>MKYPPSLVSLIRELSRLPGIGPKSAQRLAFHLFEQPREDIERLASALLEAKRDLHVCPICFNITDAEKCDVCADPSRDQRTICVVEEPGDVIALERSGEYRGLYHVLHGVLSPMNGVGPDKLHIKPLLPRVGQGMEVILATGTTVEGDATALYLQRLLEPLGAAISRIAYGVPVGGSLEYTDEVTLGRALTGRQTVSKPQPPQRPGDEDGADGAAVPASR[2x];> MRSRTANRSGIVIRRRVTPAGDIIVTLLTPQGKLKAIARGGVKGPLSSSLNLFHHVGVQVYQGPHNDLASVKQAVLEGALPTLAEPERYAFAHLMAEFADALFQEGEFSEQAFDLFAASLRG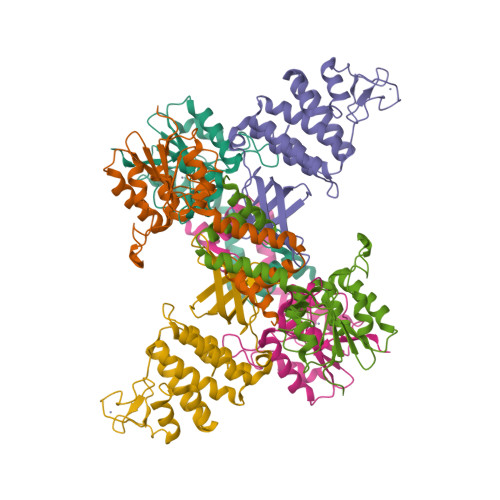VAHQPDPEWVALVMSYKLLGLAGVIPQTARCARCGAPDPEHPDPLGGQLLCSKCAALPPYPPAVLDFLRHAVRRTVRASFEQPVPSADRPALWRALEKFVTVQVGGVHSWRQLVPSGVPVLS>[4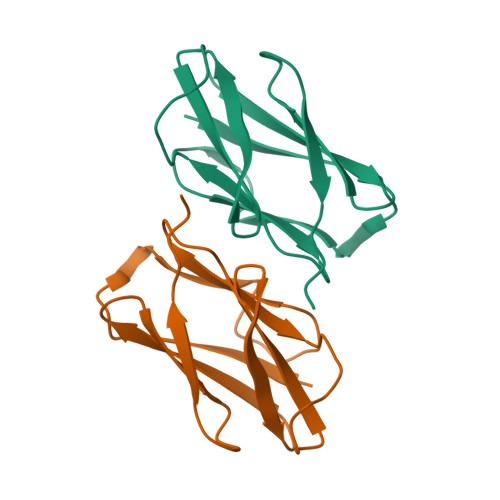x]MVWSVQIVDNAGLGANLALYPSGNSSTVPRYVTVTGYAPITFSEIGPKTVHQSWYITVHNGDDRAFQLGYEGGGVATATFTAGGNVSISTGFGDAQHLTLKKLA>[2x]MNPAAEAEFNILLATDSYKVTHYKQYPPNTSKVYSYFECREKKTENSKLRKVKYEETVFYGLQYILNKYLKGKVVTKEKIQEAKDVYKEHFQDDVFNEKGWNYILEKYDGHLPIEIKAVPEGFVIPRGNVLFTVENTDPECYWLTNWIETILVQSWYPITVATNYREQKKILAKYLLETSGNLDGLEYKLHDFGYRGVSSQETAGIGASAHLVNFKGTDTVAGLALIKKYYGTKDPVPGYSVPAAEHSTITAWGKDHEKDAFEHIVTQFSSVPVSVVSDSYDIYNACEKIWGEDLRHLIVSRSTQAPLIIRPDSGNPLDTVLKVLEILGKKFPVTENSKGYKLLPPYLRVIQGDGVDINTLQEIVEGMKQKMWSIENIAFGSGGGLLQKLTRDLLNCSFKCSYVVTNGLGINVFKDPVADPNKRSKKGRLSLHRTPAGNFVTLEEGKGDLEEYGQDLLHTVFKNGKVTKSYSFDEIRKNAQLNIELEAAHHLEHHHHHHHH

NAMPT functions as a homo-dimeric enzyme that catalyzes the rate limiting step in the primary salvage pathway for NAD synthesis, the transfer of a phosphoribosyl residue from 5-phosphoribosyl-1-pyrophosphate (PRPP) to nicotinamide (NAM) to produce nicotinamide mononucleotide (NMN). Crystal structures of NAMPT in numerous ligand-bound forms have been reported. These structures consistently display a NAMPT homo-dimer with two essentially identical active sites at the dimer interface. Typical NAMPT inhibitors were found to occupy the portion of active site responsible for NAM binding and a tunnel-shaped cavity extending from the NAM binding site. Furthermore, we determine the crystal structures of six NAMPT mutants in the apo form and in complex with various inhibitors and present a definitive model to explain the differential effects of the mutations on various structural classes of NAMPT inhibitors.

The crystal structures of NAMPT S165F/Y revealed a somewhat surprising conformational change in a small helical structural motif spans the sequence G383GGLLQ388. We designate this motif as “380GRS” to reflect its position in the primary sequence, and its glycine rich characteristic. The unwinding of the 380GRS in S165 mutants rendered the structure less compatible with the binding of PRPP. Our structural studies thus reveal that the S165 mutation modulates NAMPT activity by interfering with PRPP binding in an allosteric manner. Consistent with the structural observations, S165F/Y mutant NAMPT proteins required approximately 500 fold more PRPP compared to the wild-type protein and the other NAMPT mutants. In all cases the S165Y mutant resulted in greater resistance to NAMPT inhibitors. In contrast, NCI-H460 S165Y tumor xenografts were completely resistant to treatment with GNE-618, even when dosed daily (QD) at higher drug concentrations. Furthermore, xenografts derived from cells harboring the S165Y mutation in NAMPT are resistant to GNE-618 at doses that are efficacious in the parental line, suggesting that this is relevant in vivo.> MANVDEAILKRVKGWAPYVDAKLGFRNHWYPVMFSKEINEGEPKTLKLLGENLLVNRIDGKLYCLKDRCLHRGVQLSVKVECKTKSTITCWYHAWTYRWEDGVLCDILTNPTSAQIGRQKLKTYPVQEAKGCVFIYLGDGDPPPLARDTPPNFLDDDMEILGKNQIIKSNWRLAVENGFDPSHIYIHKDSILVKDNDLALPLGFAPGGDRKQQT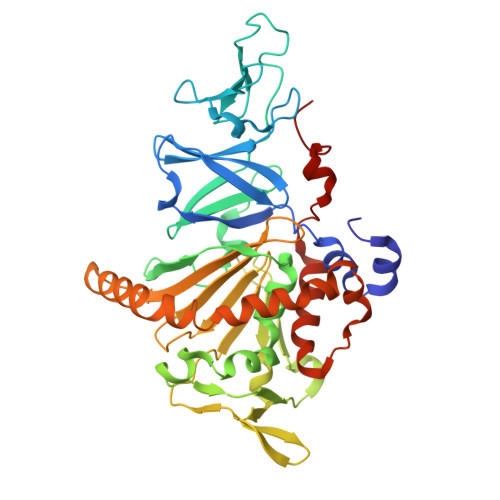RVVDDDVVGRKGVYDLIGEHGVPVFEGTIGGEVVREGAYGEKIVANDISIWLPGVLKVNPFPNPDMMQFEWYVPIDENTHYYFQTLGKPCANDEERKKYEQEFESKWKPMALEGFNNDDIWAREAMVDFYADDKGWVNEILFESDEAIVAWRKLASEHNQGIQTQAHVSGLEHHHHHH> DRRSFSSRTPVNENPDGV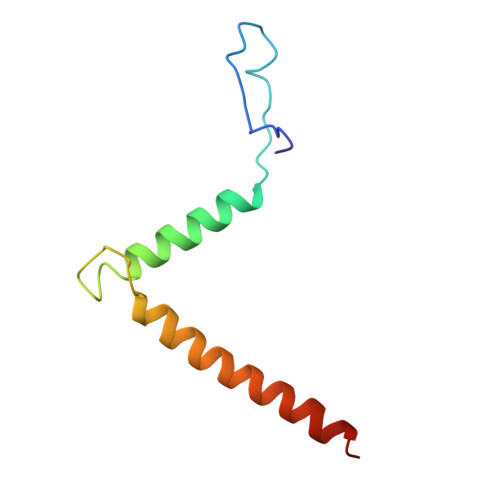QYRRGFVTRHQVSGWRFVMRRIASGVALHDTRMLVDPLRTQSRAVLTGALILVTGLVGCFIFSLF>[3x]MSLSNIETVP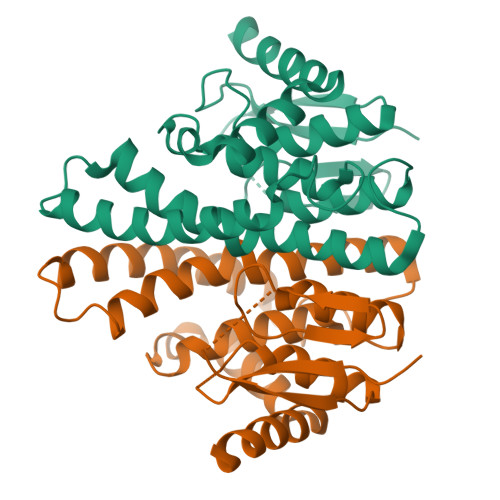ASIEMKPNPTITVFERSPDGGRGLARDMPVRWALEEVGQPYHVRRLSFEAMKEASHLAYQPFGQIPSYEQGDLILFESGAIVMHIAQHHSGLLPEDQLRRARTVAWMFAALNTIEPSILNFTTVWLFERNEPWHEARLARTKEQLLKRLDELSAWLGDREWLEGSFSAADILMICVLRRLESSGILKDYGNLLAYVERGKARPAFKRAFDAQLAVFTAASKNEGHHHHHH The endoribonuclease EndoU-like (Endoribonucleases specific for Uridylate) superfamily (IPR037227) is a poorly understood group of RNases found in bacteria, eukaryotes and viruses. Human EndoU (hEndoU) was first identified as human placental protein 11 (PP11) due to its prevalence in the placenta. EndoU showed little dependence on Na+ or K+ and sustained activity across pH 4–8. These results indicate EndoU is a calcium-activated ribonuclease targeting a large repertoire of RNAs. Our structural analysis revealed a calcium-stabilized interaction network involving residues from both the eukaryote-specific N-terminal extension and the catalytic core of EndoU, ultimately leading to the activation of the catalytic triad.

To elucidate the effect of calcium, we crystallized EndoU with an excess of calcium and solved its structure at 1.7 Å resolution. The structure revealed five calcium ions, with one aiding crystal packing and four potentially activating the protein. Each calcium ion is coordinated by seven oxygen atoms from acidic side-chains, backbone carbonyl groups, or protein-stabilized water molecules. Sites (1) and include residues from both the catalytic core and the eukaryote-specific N-terminal extension, with site (1) located 12.8 Å away from the catalytic triad (H285, H300, K343). Comparing apo-XendoU, apo-EndoU, and calcium-activated EndoU structures revealed conformational changes upon calcium binding that mainly cluster nearby protein loops. The side-chain of E290, located midway between site (1) and the catalytic triad, flips to engage with a water molecule in the calcium coordination network. This correlates with the side-chain rotation of catalytic H285, then locked by an electrostatic interaction with E290. The bonding correlates with a disorder-to-order transition in the loop carrying E290, forming a β-hairpin and stabilizing the catalytic site. Our data show a model for the calcium-dependent regulation of EndoU through allostery, with site (1) and residue E290 as key mediators in the intramolecular signaling leading to EndoU activation. Therefore, our work supports a model where calcium is not directly involved in catalysis but rather activates the catalytic His-His-Lys triad through allostery.

>[2x]MRACISLVLAVLCGLAWAGKIESCASRCNEKFNRDAACQCDRRCLWHGNCCEDYEHLCTEDHKESEPLPQLEEETEEALASNLYSAPTSCQGRCYEAFDKHHQCHCNARCQEFGNCCKDFESLCSDHEVSHSSDAITKEEIQSISEKIYRADTNKAQKEDIVLNSQNCISPSETRNQVDRCPKPLFTYVNEKLFSKPTYAAFINLLNNYQRATGHGEHFSAQELAEQDAFLREIMKTAVMKELYSFLHHQNRYGSEQEFVDDLKNMWFGLYSRGNEEGDSSGFEHVFSGEVKKGKVTGFHNWIRFYLEEKEGLVDYYSHIYDGPWDSYPDVLAMQFNWDGYYKEVGSAFIGSSPEFEFALYSLCFIARPGKVCQLSLGGYPLAVRTYTWDKSTYGNGKKYIATAYIVSST>GGSGQPDMSLNVIKMKSSDFLESAELDSGGFGKVSLAFHRTQGLMIMKTVYKGPNCIEHNEALLEEAKMMNRLRHSRVVKLLGVIIEEGKYSLVMEYMEKGNLMHVLKAEMSTPLSVKGRIILEIIEGMAYLHGKGVIHKDLKPENILVDNDFHIKIADLGLASFKMWSKLNNEEHNE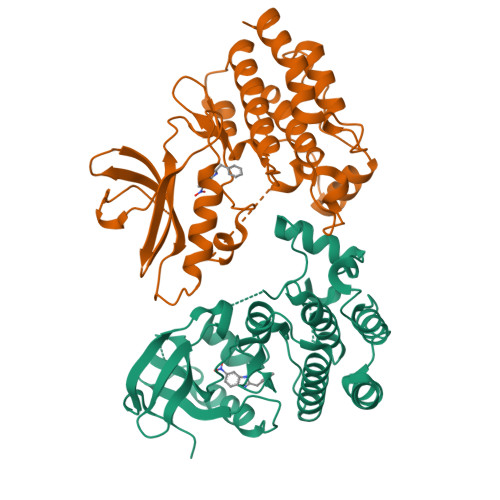LREVDGTAKKNGGTLYYMAPEHLNDVNAKPTEKSDVYSFAVVLWAIFANKEPYENAIAEQQLIMAIKSGNRPDVDDLTEYCPREIISLMKLCWEANPEARPTFPGIEEKFRPFYLSQLE[2x]> MQDNSRYTHFLTQHYDAKPQGRDDRYCESIMRRRGLTSPCRDINTFIHGNKRSIKAICENKNGNPHRENLRISKSSFQVTTCKLHGGSPWPPCQYRATAGFRNVVVACENGLPVHLDQSIFRRP

Angiogenin (ANG), a 14-kDa basic protein is an angiogenic ribonuclease and member of the bovine pancreatic ribonuclease (RNase A) family (also known as RNase 5). Like RNase A, ANG cleaves preferentially on the 3′ side of pyrimidines and follows a transphosphorylation/hydrolysis mechanism. In addition, the crystal structure of human ANG has revealed that it has an RNase A fold and the catalytic triad (residues H13, K40 and H114) is conserved. The enzymatic activity of ANG is several orders of magnitude lower than that of RNase A towards conventional RNase substrates, but essential for its angiogenic effect.

ANG residues H13, K40 and H114 (part of the P1 sub-site) correspond to the catalytic triad. K40 is a key residue at the catalytic centre of ANG and adopts multiple conformation in the native structure. However the conservative substitution of Arg for K40 reduces the activity to ~6%, similar to the effect of the K41 to Arg mutation in RNase A43. In the crystal structure of the ALS variant K40R, the Arg side chain possesses a single conformation and several key interactions of K40 (with residues Q12, C39, N43 and T44, which are integral to the catalytic site) known to be important for the stabilization of the pentavalent transition state during RNA cleavage are lost. Instead, in the variant, the Arg side-chain makes direct interaction with Q112 by reorienting its side chain (more solvent exposed).> MNAVEIISREISPTLDIQTKILEYMTDFFVKEGFKWLLPVIISPITDPLWPDPAGEGMEPAEVEIYGVKMRLTHSMILHKQLAIAMGLKKIFVLSPNIRLESRQKDDGRHAYEFTQLDFEVERAKMEDIMRLIERLVYGLFRKAEEWTGREFPKTKRFEVFEYSEVLEEFGSDEKASQEMEEPFWIINIPREFYDREVDGFWRNYDLILPYGYGEVASGGEREWEYEKIVAKIRKA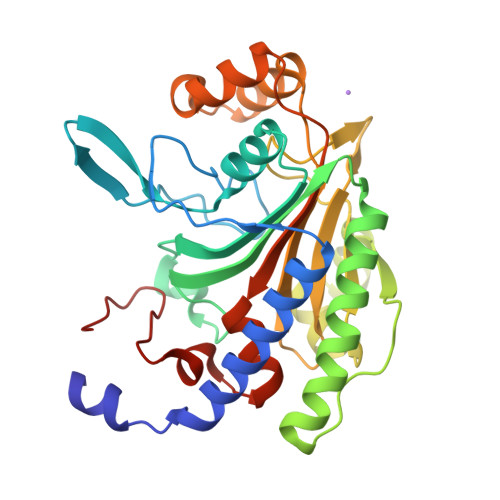GLNEDSFRPYLEIAKAGKLKPSAGAGIGVERLVRFIVGAKHIAEVQPFPRIPGIPAVI methyl (3~{S},7~{R},10~{R},13~{R})-4-[(3~{S},6~{R},8~{a}~{S})-1'-[(2~{S})-2-acetamido-3-(2-chlorophenyl)propanoyl]-5-oxidanylidene-spiro[1,2,3,8~{a}-tetrahydroindolizine-6,2'-pyrrolidine]-3-yl]carbonyl-2-oxidanylidene-1,4-diazatricyclo[8.3.0.0^{3,7}]tridec-8-ene-13-carboxylate 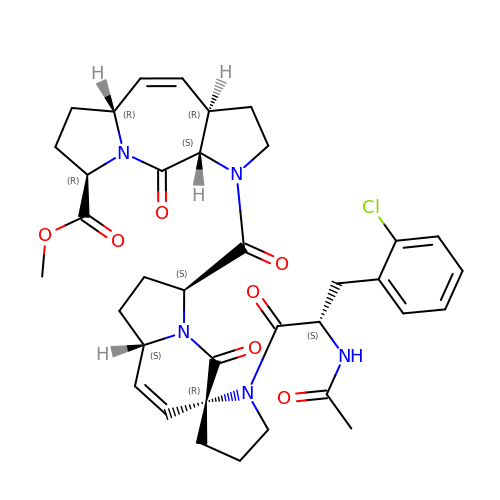| C36 H42 Cl N5 O7 | GZPHGKMETPUDJS-UIJLVBHGSA-N> GDVTFDVGDEYEIIETIGNGAYGVVSSARRRLTGQQVAIKKIPNAFDVVTNAKRTLRELKILKHFKHDNIIAIKDILRPTVPYGEFKSVYVVLDLMESDLHQIIHSSQPLTLEHVRYFLYQLLRGLKYMHSAQVIHRDLKPSNLLVNENCELKIGDFGMARGLCTSPAEHQYFMTEYVATRWYRAPELMLSLHEYTQAIDLWSVGCIFGEMLARRQLFPGKNYVHQLQLIMMVLGTPSPAVIQAVGAERVRAYIQSLPPRQPVPWETV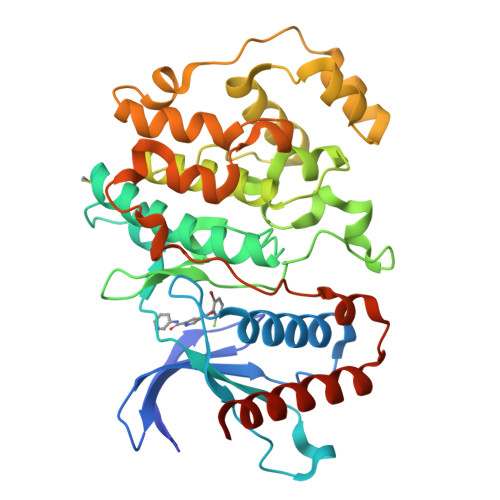YPGADRQALSLLGRMLRFEPSARISAAAALRHPFLAKYHDPDDEPDCAPPFDFAFDREALTRERIKEAIVAEIEDFHARREGIRQQIRFQ>[2x]VPSSALSEV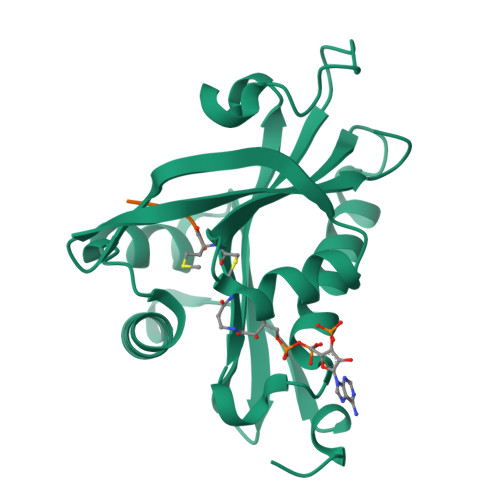SLRLLCHDDIDTVKHLCGDWFPIEYPDSWYRDITSNKKFFSLAATYRGAIVGMIVAEIKNRTKIHKEDGDILASNFSVDTQVAYILSLGVVKEFRKHGIGSLLLESLKDHISTTAQDHCKAIYLHVLTTNNTAINFYENRDFKQHHYLPYYYSIRGVLKDGFTYVLYINGG;>MKAV[2x]>[6x]MGSSHHHHHHGGGSENLYFQGCSDIWALQGKSTETNPLYWLRAMDCADRLMPAQSRQQARQYDDGSWQNTFKQGILLADAKITPYERRQLVA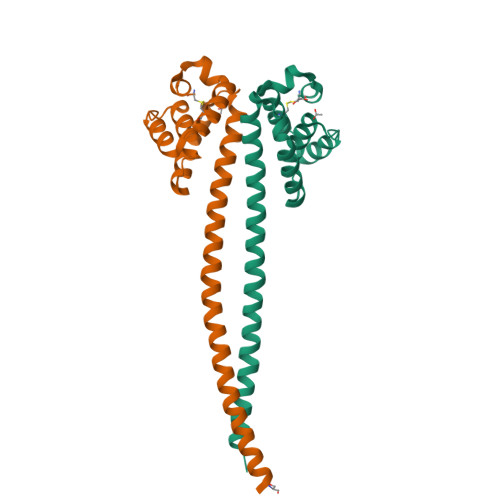RIEALSTEIPAQVRPLYQLWRDGQALQLQLAEERQRYSKLQQSSDSELDTLRQQHHVLQQQLELTTRKLENLTDIERQLSTRK>[4x]ADLKVGFITSLSGPVSSLGIPYEKGMKAAIAYKSDVGGRKIQLVQLDDASDPSTAARNARKMIDEDKVDVIIGTAGSPGALAIAGVARETKTPLISIANANLPGEEGAWMVTLPQPAPLMVSAVVERMKKSGVKTVGYIGFSDAWGDLVYDALQKSAEPAGIKIVSNERYARADSSVTGQVL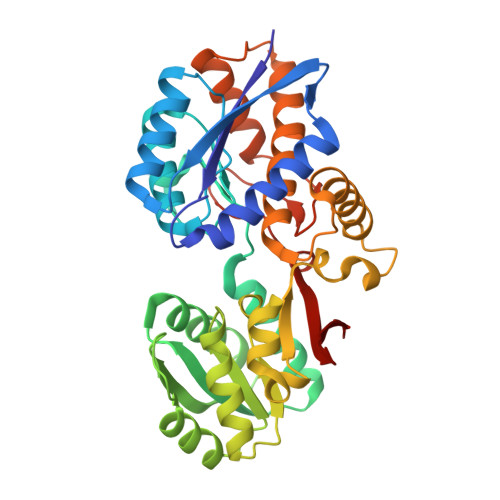KIVALRPDAVITGTSGTPGALPYLALAERGYKGQIYGMHALINPDFVRVGGASVEGLLAPTGPVIVAEQLPSENPIRKVSMDFRAAYQKANGAPPTDAFSAYTFDAWLLYLDAAQRALATKAEPGTPQFRLALRDAIVSTKELVGTHSVYNFKPTDRYGSDERSRVVVKLEKGQWKLVK>HHHHHHGSMDKNIIIGAMTALITPFKNGKVDEQSYARLIKRQIENGIDAVVPVGTTGESATLTHEEHRTCIEIAVETCKGTKVKVLAGAGSNATHEAVGLAKFAKEHGADGILSVAPYYNKPTQQGLYEHYKAIAQSVDIPVLLYNVPGRTGCEISTDTIIKLFRDCENIYGVKEASGNIDKCVDLLAHEPRMMLISGEDAINYPILSNGGKGVISVTSNLLPDMISALTHFALDENYKEAKKINDELYNINKILFCESNPIPIKTAM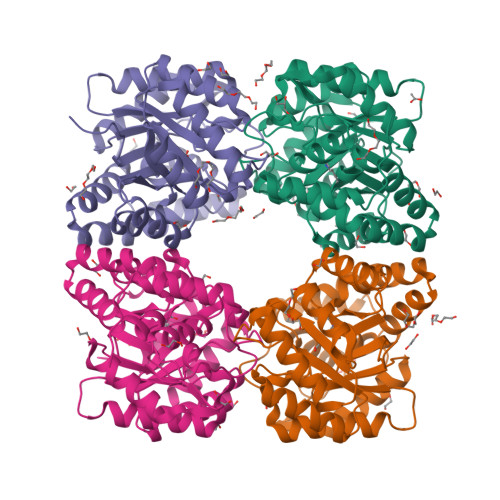YLAGLIESLEFRLPLCSPSKENFAKIEEVMKKYKIKGF[4x]> MAPSRLCVYCADVCPDRLRCAAWLLATGIFLLLAGCSEAKAPTALERVQKEGVLRVITRNSPATYFQDRNGETGFEYELAKRFAERLGVELKIETADNLDDLYAQLSREGGPALAAAGLTPGREDDASVRYSHTYLDVTPQIIYRNGQQRPTRPEDLVGKRIMVLKGSSHAEQLAELKKQYPELKYEESDAVEVVDLLRMVDVGDIDLTLVDSNELAMNQVYFPNVRVAFDFGEARGLAWALPGGDDDSLMNEVNAFLDQAKKEGLLQRLKDRYYGHVDVLGYVGAYTFTQHLQQRLPRYESHFKQSGKQKDTDWRLLAAIGYQESLWQPGATSKTGVRGLMMLTNRTAQAMGVSNRLDPKQSIQGGSKYFVQIRSELPESIKEPDRSWFALAAYNIGGAHLEDARKMAEKEGLNPNKWLD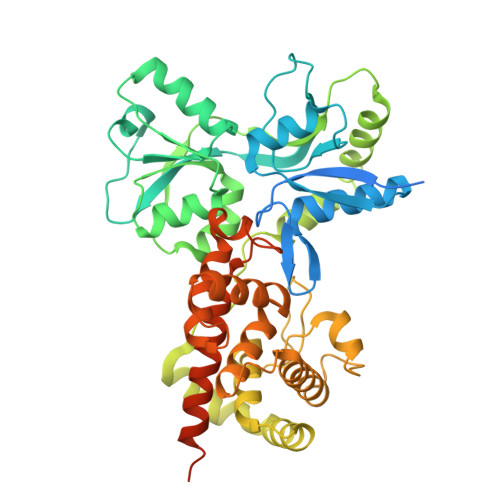VKKMLPRLAQKQWYAKTRYGYARGGETVHFVQNVRRYYDILTWVTQPQMEGSQIAESGLHLPGVNKTRPEEDSGDEKL> MTLSILVAHDLQR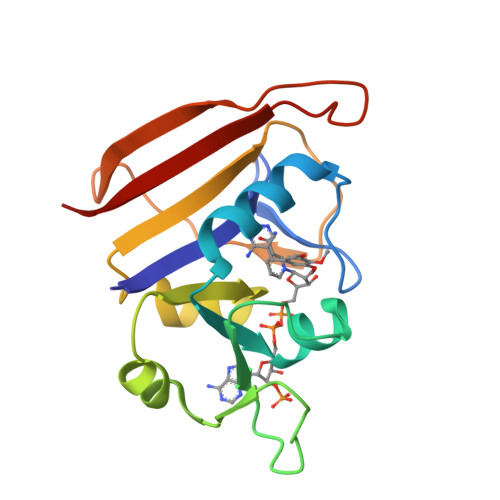VIGFENQLPWHLPNDLKHVKKLSTGHTLVMGRKTFESIGKPLPNRRNVVLTSDTSFNVEGVDVIHSIEDIYQLPGHVFIFGGQTLFEEMIDKVDDMYITVIEGKFRGDTFFPPYTFEDWEVASSVEGKLDEKNTIPHTFLHLIRKK8-{2-[2-(2,4-dioxo-3,4-dihydropyrimidin-1(2H)-yl)ethoxy]-4-fluorophenoxy}-6-fluoroindolizine-2-carbonitrile 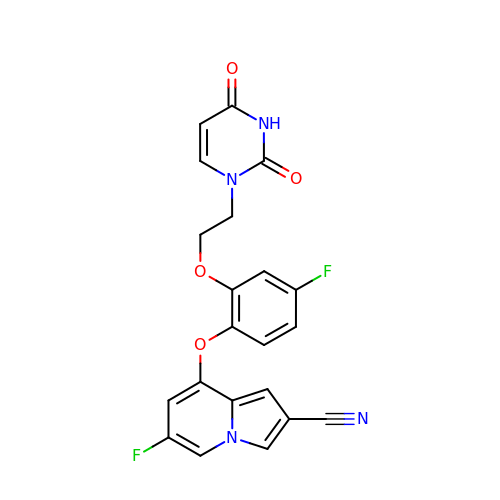| C21 H14 F2 N4 O4 | ZZRRYEXYIVBDNM-UHFFFAOYSA-N>DAMVKYEELLKTLENGINSEEGEIRLVRKSQGRFKEEFNFDLSLGSKPLLTLKVFLGRKPYWQPWVEVFGVNPNLRNVFFGS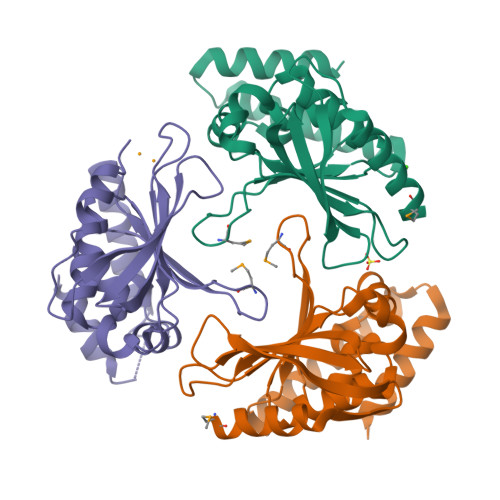EAERKLYEFLSEHFGRIFVEYFEDKETTYELQKGVPPALSRLGFELLKLGYTYFRDWFIPEGLMEGGHKIQAEKPKTEEAKKRHLENLKKEFEEFIGKCEDEGLIKKVKERYNFLEHEGSS[3x]>[2x]MAK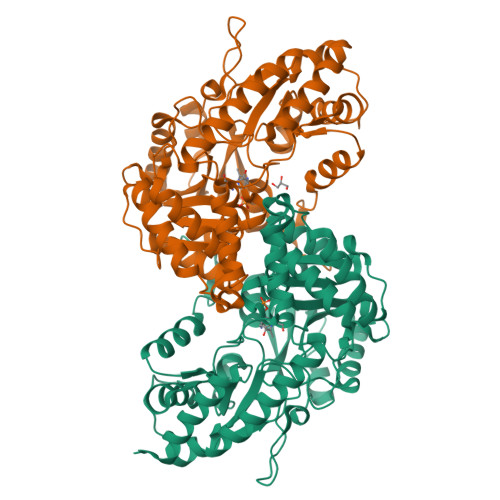QLQARRLDGIDYNPWVEFVKLASEHDVVNLGQGFPDFPPPDFAVEAFQHAVSGDFMLNQYTKTFGYPPLTKILASFFGELLGQEIDPLRNVLVTVGGYGALFTAFQALVDEGDEVIIIEPFFDCYEPMTMMAGGRPVFVSLKPGPIQNGELGSSSNWQLDPMELAGKFTSRTKALVLNTPNNPLGKVFSREELELVASLCQQHDVVCITDEVYQWMVYDGHQHISIASLPGMWERTLTIGSAGKTFSATGWKVGWVLGPDHIMKHLRTVHQNSVFHCPTQSQAAVAESFEREQLLFRQPSSYFVQFPQAMQRCRDHMIRSLQSVGLKPIIPQGSYFLITDISDFKRKMPDLPGAVDEPYDRRFVKWMIKNKGLVAIPVSIFYSVPHQKHFDHYIRFCFVKDEATLQAMDEKLRKWKVEL>PSVYDAAAQLTADVKKDLRDSWKVIGSDKKGNGVALVTTLFADNQETIGYFKRLGDVSQGMANDKLRGHSITIMYALQNFIDQLDNPDDLVCVVEKFAVNHITRKISAAEFGKINGPIKKVLASKNFGD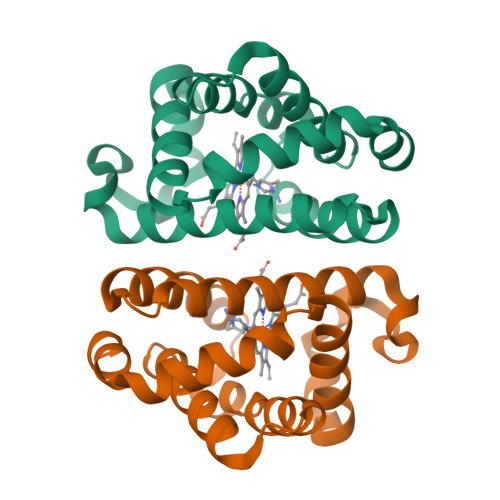KYANAWAKLVAVVQAAL[2x]>[14x]AEPVYPDQLRLFSLGQGVCGDKYRPVNREEAQSVKSNIVGMMGQWQISGLANGWVIMGPGYNGEIKPGTASNTWCYPTNPVTGEIPTLSA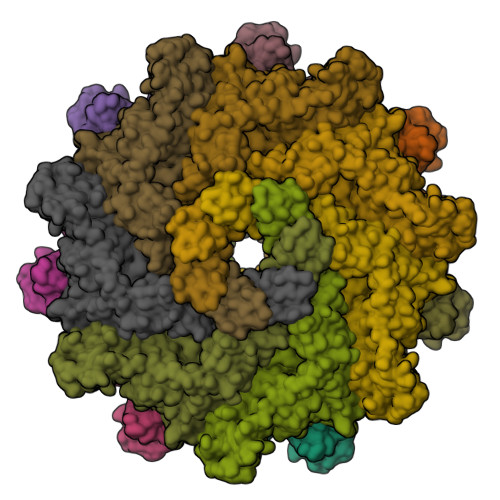LDIPDGDEVDVQWRLVHDSANFIKPTSYLAHYLGYAWVGGNHSQYVGEDMDVTRDGDGWVIRGNNDGGCDGYRCGDKTAIKVSNFAYNLDPDSFKHGDVTQSDRQLVKTVVGWAVNDSDTPQSGYDVTLRYDTATNWSKTNTYGLSEKVTTKNKFKWPLVGETALSIAIAANQSWASQNGGSTTTSLSQSVRPTVPARSKIPVKIELYKADISYPYEFKADVSYDLTLSGFLRWGGNAWYTHPDNRPNWNHTFVIGPYKDKASSIRYQWDKRYIPGEVKWWDWNWTIQQNGLSTMQNNLARVLRPVRAGITGDFSAESQFAGNIEIGAPVPLAA> MENMFSLQGKIALITGASYGIGFEIAKAYAQAGATIVFNDIKQELVDKGLAAYRELGIEAHGYVCDVTDEAGIQQMVSQIE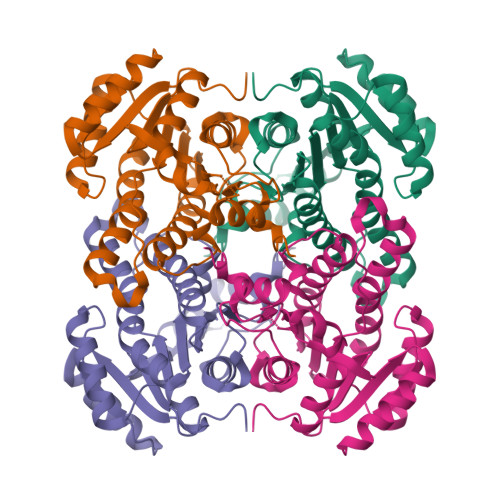DEVGAIDILVNNAGIIRRTPMLEMAAEDFRQVIDIDLNAPFIVSKAVLPSMIAKGHGKIINICSMMSELGRETVSAYAAAKGGLKMLTKNIASEFGEANIQCNGIGPGYIATPQTAPLRERQADGSRHPFDQFIIAKTPAARWGTTEDLAGPAVFLASDASNFVNGHILYVDGGILAYIGKQP As a scaffold for aromatic cluster design, we chose ferritin as a protein cage platform with a 12 nm outer diameter and an 8 nm inner cavity, composed of 24 subunits. To prove this concept through protein engineering, we focused on a two‐fold symmetric inter‐subunit interface of a recombinant horse spleen apo‐L ferritin (Fr) as a target region for mutagenesis. Herein, we present the construction of an aromatic cluster with an artificial molecular binding pocket at the two‐fold symmetric interface of ferritin and explore its ligand‐binding characteristics. We developed a system that uses ligand binding as a driving force to induce and propagate changes in the orientation of multiple aromatic side chains.

Next, we replaced Glu residues located near residue 59 with Phe residues to form an aromatic cluster surrounding the Phe59 pocket. The resulting mutants were named Fr‐F2 (Fr‐E56F/R59F), Fr‐F4 (Fr‐R52F/E56F/R59F/E63F), and Fr‐F6 (Fr‐E53F/E56F/E57F/R59F/E60F/E63F), where i in Fr‐Fi represents the number of newly introduced Phe residues per ferritin monomer (upper). Analysis of the 2Fo‐Fc maps revealed electron densities corresponding to Nile Red (NR) at the two‐fold symmetric interfaces of NR•Fr‐F1, NR•Fr‐F2, NR•Fr‐F4, and NR•Fr‐F6, observed as overlapping densities due to the interface symmetry. NR was positioned between two F59 residues, forming π–π stacking interactions in an F59–NR–F59' configuration. Anion‐π interactions between NR and E60 in NR•Fr‐F1 and NR•Fr‐F2, and CH‐π interactions between NR and F60 in NR•Fr‐F6, were identified, indicating NR's stabilization in the F59–F59' pocket via multiple non‐covalent interactions. Notably, NR•Fr‐F1 and NR•Fr‐F2, containing only one and two Phe residues, respectively, achieve higher quantum yields (94 and 95%, respectively) and longer lifetimes (5.54 and 5.75 ns, respectively) than NR•Fr‐F6 with six Phe residues per monomer. The hydrophobic and polar nature of the protein surface around NR influences its fluorescence properties, with the partially polar microenvironment in Fr‐F1 and Fr‐F2, attributed to Glu residues near the pocket entrance, potentially enhancing fluorescence.

> SSQIRQNYSTEVEAAVNRLVNLYLRASYTYLSLGFYFDRDDVALEGVCHFFRELAFEKFEGAERLLKMQNQRGGRALFQDLQKPSQDEWGTTLDAMKAAIVLEKSLNQALLDLHALGSAQADPHLCDFLESHFLDEEVKLIKKMGDHLTNIQRLVGSQAGLGEYLFERLTLKHD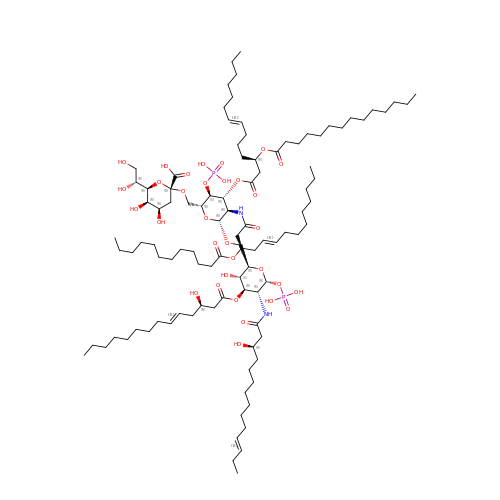(2~{R},4~{R},5~{R},6~{R})-6-[(1~{R})-1,2-bis(oxidanyl)ethyl]-2-[[(2~{R},3~{S},4~{R},5~{R},6~{R})-5-[[(~{E},3~{R})-3-dodecanoyloxytetradec-5-enoyl]amino]-6-[[(2~{R},3~{S},4~{R},5~{R},6~{R})-3-oxidanyl-5-[[(~{E},3~{R})-3-oxidanyltetradec-11-enoyl]amino]-4-[(~{E},3~{R})-3-oxidanyltetradec-5-enoyl]oxy-6-phosphonooxy-oxan-2-yl]methoxy]-3-phosphonooxy-4-[(~{E},3~{R})-3-tetradecanoyloxytetradec-7-enoyl]oxy-oxan-2-yl]methoxy]-4,5-bis(oxidanyl)oxane-2-carboxylic acid | C102 H182 N2 O32 P2 | NOEIKEOYYQLMFH-XTQPGWFYSA-N> MAAQVTLEDALSNVDLLEELPLPDQQPCIEPPPSSLLYQPNFNTNFEDRNAFVTGIARYIEQATVHSSMNEMLEEGQEYAVMLYTWRSCSRAIPQVKCNEQPNRVEIYEKTVEVLEPEVTKLMNFMYFQRNAIERFCGEVRRLCHAERRKDFVSEAYLITLGKFINMFAVLDELKNMKCSVKNDHSAYKRAAQFLRKMADPQSIQESQNLSMFLANHNKITQSLQQQLEVISGYEELLADIVNLCVDYYENRMYLTPSEKHMLLKVMGFGLYLMDGSVSNIYKLDAKKRINLSKIDKYFKQLQVVPLFGDMQIELARYIKTSAHYEENKSRWTCTSSGSSPQYNICEQMIQIREDHMRFISELARYSNSEVVTGSGRQEAQKTDAEYRKLFDLALQGLQLLSQWSAHVMEVYSWKLVHPTDKYSNKDCPDSAEEYERATRYNYTSEEKFALVEVIAMIKGLQVLMGRMESVFNHAIRHTVYAALQDFSQVTLREPLRQAIKKKKNVIQSVLQAIRKTVCDWETGHEPFNDPALRGEKDPKSGFDIKVPRRAVGPSSTQLYMVRTMLESLIADKSGSKKTLRSSLEGPTILDIEKFHRESFFYTHLINFSETLQQCCDLSQLWFREFFLELTMGRRIQFPIEMSMPWILTDHILETKEASMMEYVLYSLDLYNDSAHYALTRFNKQFLYDEIEAEVNLCFDQFVYKLADQIFAYYKVMAGSLLLDKRLRSECKNQGATIHLPPSNRYETLLKQRHVQLLGRSIDLNRLITQRVSAAMYKSLELAIGRFESEDLTSIVELDGLLEINRMTHKLLSRYLTLDGFDAMFREANHNVSAPYGRITLHVFWELNYDFLPNYCYNGSTNRFVRTVLPFSQEFQRDKQPNAQPQYLHGSKALNLAYSSIYGSYRNFVGPPHFQVICRLLGYQGIAVVMEELLKVVKSLLQGTILQYVKTLMEVMPKICRLPRHEYGSPGILEFFHHQLKDIVEYAELKTVCFQNLREVGNAILFCLLIEQSLSLEEVCDLLHAAPFQNILPRVHVKEGERLDAKMKRLESKYAPLHLVPLIERLGTPQQIAIAREGDLLTKERLCCGLSMFEVILTRIRSFLDDPIWRGPLPSNGVMHVDECVEFHRLWSAMQFVYCIPVGTHEFTVEQCFGDGLHWAGCMIIVLLGQQRRFAVLDFCYHLLKVQKHDGKDEIIKNVPLKKMVERIRKFQILNDEIITILDKYLKSGDGEGTPVEHVRCFQPPIHQSLASS;> MSRSVLQPSQQKLAEKLTILNDRGVGMLTRLYNIKKACGDPKAKPSYLIDKNLESAVKFIVRKFPAVETRNNNQQLAQLQKEKSEILKNLALYYFTFVDVMEFKDHVCELLNTIDVCQVFFDITVNFDLTKNYLDLIITYTTLMILLSRIEERKAIIGLYNYAHEMTHGASDREYPRLGQMIVDYENPLKKMMEEFVPHSKSLSDALISLQMVYPRRNLSADQWRNAQLLSLISAPSTMLNPAQSDTMPCEYLSLDAMEKWIIFGFILCHGILNTDATALNLWKLALQSSSCLSLFRDEVFHIHKAAEDLFVNIRGYNKRINDIRECKEAAVSHAGSMHRERRKFLRSALKELATVLSDQPGLLGPKALFVFMALSFARDEIIWLLRHADNMPKKSADDFIDKHIAELIFYMEELRAHVRKYGPVMQRYYVQYLSGFDAVVLNELVQNLSVCPEDESIIMSSFVNTMTSLSVKQVEDGEVFDFRGMRLDWFRLQAYTSVSKASLGLADHRELGKMMNTIIFHTKMVDSLVEMLVETSDLSIFCFYSRAFEKMFQQCLELPSQSRYSIAFPLLCTHFMSCTHELCPEERHHIGDRSLSLCNMFLDEMAKQARNLITDICTEQ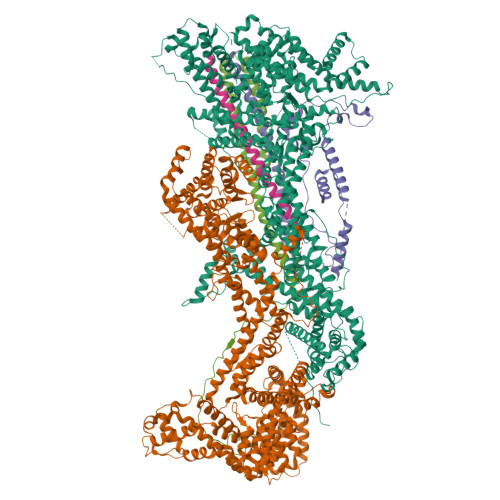CTLSDQLLPKHCAKTISQAVNKKSKKQTGKKGEPEREKPGVESMRKNRLVVTNLDKLHTALSELCFSINYVPNMVVWEHTFTPREYLTSHLEIRFTKSIVGMTMYNQATQEIAKPSELLTSVRAYMTVLQSIENYVQIDITRVFNNVLLQQTQHLDSHGEPTITSLYTNWYLETLLRQVSNGHIAYFPAMKAFVNLPTENELTFNAEEYSDISEMRSLSELLGPYGMKFLSESLMWHISSQVAELKKLVVENVDVLTQMRTSFDKPDQMAALFKRLSSVDSVLKRMTIIGVILSFRSLAQEALRDVLSYHIPFLVSSIEDFKDHIPRETDMKVAMNVYELSSAAGLPCEIDPALVVALSSQKSENISPEEEYKIACLLMVFVAVSLPTLASNVMSQYSPAIEGHCNNIHCLAKAINQIAAALFTIHKGSIEDRLKEFLALASSSLLKIGQETDKTTTRNRESVYLLLDMIVQESPFLTMDLLESCFPYVLLRNAYHAVYKQSVTSSA;> MPLVKRNIDPRHLCHTALPRGIKNELECVTNISLANIIRQLSSLSKYAEDIFGELFNEAHSFSFRVNSLQERVDRLSVSVTQLDPKEEELSLQDITMRKAFRSSTIQDQQLFDRKTLPIPLQETYDVCEQPPPLNILTPYRDDGKEGLKFYTNPSYFFDLWKEKMLQDTEDKRKEKRKQKQKNLDRPHEPEKVPRAPHDRRREWQKLAQGPELAEDDANLLHKHIEVANGGGSGGSGGSGGSGGSGGSKRHPSTLPVISDARSVLLEAIRKGIQLRKVEEQREQEAKHERIENDVATILSRRIAVEYSDSEDDSEFDEVDWLE;> MAGQEDPVQREIHQDWANREYIEIITSSIKKIADFLNSFDMSCRSRLATLNEKLTALERRIEYIEARVTKGETLT;> MAELQMLLEEEIPGGRRALFDSYTNLERVADYCENNYIQSADKQRALEETKAYTTQSLASVAYLINTLANNVLQMLDIQASQLRRMESSINHISQTVDIHKEKVARREIGILTTNKNTSRTHKIIAPANLERPVRYIRKPIDYTILDDIGHGVKVSTQ>[2x]MAHHHHHHMRTSQYLLSTLKETPADAVVISHQLLLRAGMIRRLASGLYTWLPMGLRVLRKVETIVREEMNAAGALEVLMPAVQPAELWQESGRWEQYGPELLRLKDRHEREFCVGPTHEEVITDLARNELNSYKQLPINFYQIQTKFRDEIRPRFGLMRGREFIMKDAYSFHLSQDS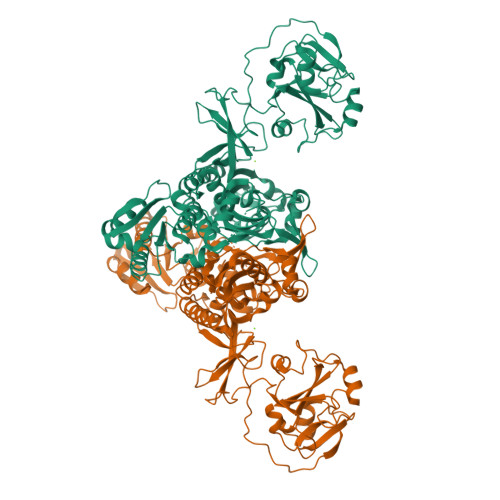LQQTYDGMYQAYSKIFSRLGLDFRPVQADNGSIGGSGSHEFHVLANSGEDDIVFSDSSDYAANIEKAEAVPRESARGSATEDMRLVDTPNTKTIAALVDGFQLPIEKTIKTLVVHGAEEGTLVALIVRGDHELNEIKAANQPLVASPLVFASEAEIRAAIGAGPGSLGPVNLPIACIVDRSVALMSDFAAGANIEDKHYFGVNWERDLPLPEVADLRNVVEGDPSPDGKGTLVIKRGIEVGHIFQLGTKYSEAMKLSVLSEQGKPVNLIMGCYGIGVSRVVAAAIEQNHDERGILWPSALAPFQIALVPLKYETESVKQATDKLYAELTAAGFEVLLDDRDKKTSPGVKFADMELIGIPHRIVISDRGLSEGVLEYKGRRDSESQNLPIGELMSFITEKLSR6-amino-4-(2-aminoethyl)-2-(methylamino)-1,7-dihydro-8H-imidazo[4,5-g]quinazolin-8-one | C12 H15 N7 O | 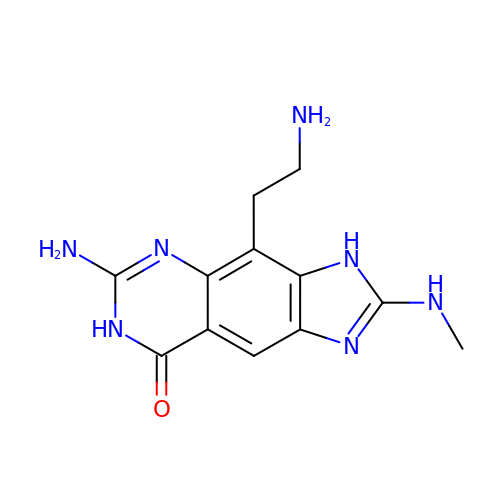GERXMHCMTFTAGY-UHFFFAOYSA-N> MDSAKLIFINQINDCKDGQKLRFLGCVQSYKNGILRLIDGSSSVTCDVTVVLPDVSIQK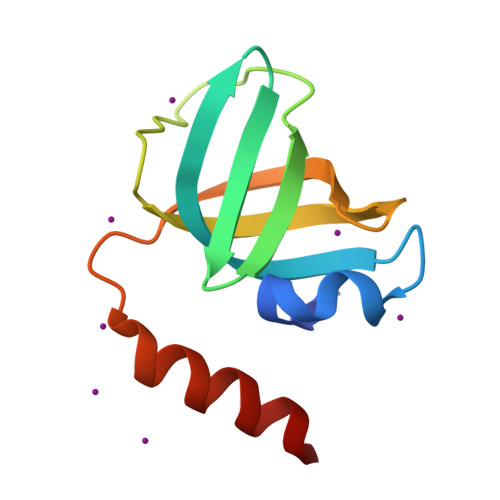HEWLNIVGRKRQDGIVDVLLIRSAVGINLPRYRQMVSERQKCD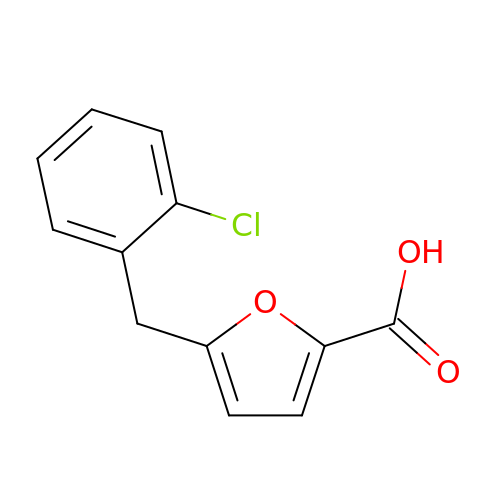5-(2-CHLOROBENZYL)-2-FUROIC ACID | C12 H9 Cl O3 | YRUPEIZURHOLHV-UHFFFAOYSA-N Cedar virus (CedV) is a Henipavirus species isolated from the excreta of Pteropus bat colonies in Queensland, Australia. HNV-G proteins comprise a short N-terminal cytosolic region, single-pass transmembrane domain, oligomerization-mediating and fusion-activating stalk region, and C-terminal receptor-binding β-propeller domain. Binding of the HNV-G to cell surface receptors belonging to the ephrin ligand family initiates pH-independent activation of F, triggering a fusion cascade that results in the ultimate merger of viral and cellular membranes. In our integrated structural and functional analysis, we demonstrate that in addition to using the common HNV receptor, ephrin-B2, CedV uses ephrin-B1, a receptor with no precedent of HNV usage.

To assess the extent to which this sequence divergence is reflected at a structural level, we determined the crystal structure of the CedV-G receptor-binding domain to 2.78-Å resolution. Electron density permitted modelling of the entire receptor-binding domain of CedV-G included in the crystallized construct (residues K209–C622). The receptor-binding domain of CedV-G adopts the canonical six-bladed β-propeller fold used by known HNVs. Each of the six blades (β1–β6) comprise four antiparallel β-strands that assemble in a toroidal arrangement and form a central depression at the membrane-distal “top” surface of the molecule. Like the prototypic HNVs, the β2 and β3 blades are decorated with extended loops that form three short 310 helical segments (η1–η3) and three α-helices (α1–α3). Eight disulphide bonds stabilize the fold, seven of which are conserved amongst other HNV-G proteins, indicative of structural importance in stabilizing the β-propeller. The additional disulphide linkage in CedV-G (C310–C376) links blades β2 and β3 at the base of the molecule. The receptor-binding domain of CedV-G possesses eight N-linked glycosylation sequons, three more than the prototypic HNV-Gs. Electron density corresponding to an asparagine-linked N-acetylglucosamine moiety was observed at seven sites. Concomitant with genetic proximity, structure-based phylogenetic classification places CedV-G in a cluster of ephrin-tropic HNV-G proteins, closer to the Asiatic prototype viruses HeV-G and NiV-G than the African GhV-G.

>ETGKIFCKSVSKDPDFRLKQIDYVIPVQQDRSICMNNPLLDISDGFFTYIHYEGINSCKKSDSFKVLLSHGEIVDRGDYRPSLYLLSSHYHPYSMQVINCVPVTCNQSSFVFCHISNNTKTLDNSDYSSDEYYITYFNGIDRPKTKKIPINNMTADNRYIHFTFSGGGGVCLGEEFIIPVTTVINTDVFTHDYCESFNCSVQTGKSLKEICSESLRSPTNSSRYNLNGIMIISQNNMTDFKIQLNGITYNKLSFGSPGRLSKTLGQVLYYQSSMSWDTYLKAGFVEKWKPFTPNWMNNTVISRPNQGNCPRYHKCPEICYGGTYNDIAPLDLGKDMYVSVILDSDQLAENPEITVFNSTTILYKERVSKDELNTRSTTTSCFLFLDEPWCISVLETNRFNGKSIRPEIYSYKIPKYCGTKHHHHHH[2x]(~{Z})-~{N}-[(~{E},2~{S},3~{R})-1-[(2~{R},3~{R},4~{S},5~{R},6~{R})-6-(hydroxymethyl)-3,4,5-tris(oxidanyl)oxan-2-yl]oxy-3-oxidanyl-octadec-4-en-2-yl]octadec-9-enamide 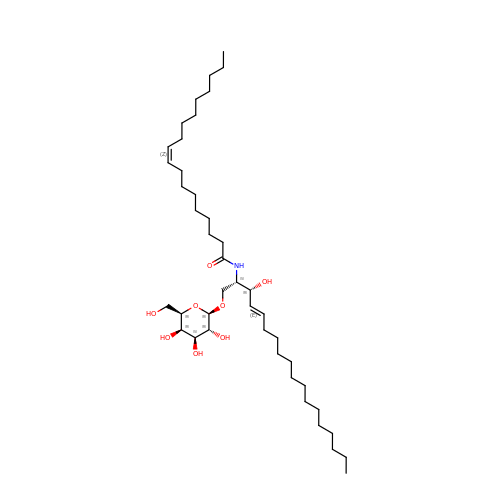| C42 H79 N O8 | MVGFIPNJBNBHNC-VTRIZHIOSA-N4-chloro-N-{[1-(3-chlorobenzene-1-carbonyl)-1,2,3,4-tetrahydroquinolin-6-yl]methyl}benzamide | 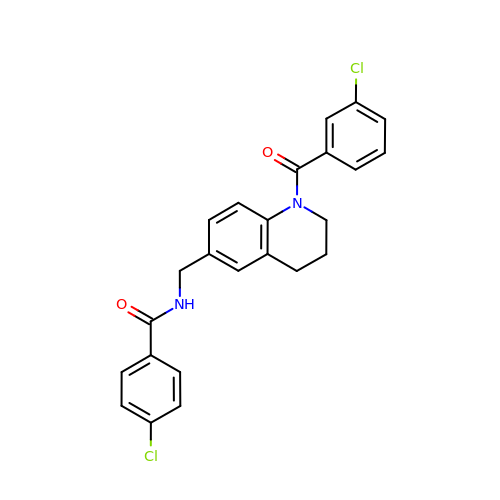C24 H20 Cl2 N2 O2 | XCOPXJUWALYDIJ-UHFFFAOYSA-N> GMEPLKVEKFATANRGNGLRAVTPLRPGELLFRSDPLAYTVCKGSRGVVCDRCLLGKEKLMRCSQCRVAKYCSAKCQKKAWPDHKRECKCLKSCKPRYPPDSVRLLGRVVFKLMDGAPSESEKLYSFYDLESNINKLTEDRKEGLRQLVMTFQHFMREEIQDASQLPPAFDLFEAFAKVICNSFTICNAEMQEVGVGLYPSISLLNHSCDPNCSIVFNGPHLLLRAVRDIEVGEELTICYLDMLMTSEERRKQLRDQYCFECDCFRCQTQDKDADMLTGDEQVWKEVQESLKK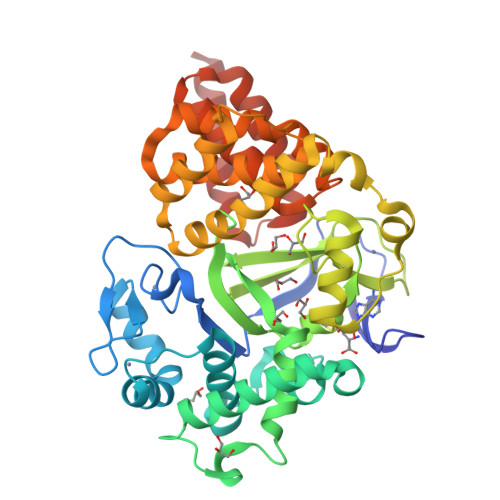IEELKAHWKWEQVLAMCQAIISSNSERLPDINIYQLKVLDCAMDACINLGLLEEALFYGTRTMEPYRIFFPGSHPVRGVQVMKVGKLQLHQGMFPQAMKNLRLAFDIMRVTHGREHSLIEDLILLLEECDANIRAS> MATRLDRLVTILETGSTRLIRDTAVNQLADWQKQHPEELFNLLSRVVPYLRHKDWETRTTAAKAIGKIIENAPLYDPNAGQDEAAPEPTNGSFEVKKEEEKDVLEQDNFFRLESLDVATIVKYGRPLLRGGPVDYNLAALDPQKRLAHLKKTLNGRLGLLGRVFEDEEMPVEQIASPITPNDAAGANGVGRQDGASNDNQSQAIDESKMSARQLNVLKRKRKREAQKAAQGKSGFGDLSLRRSTTAGSDAFGEDTPMPDADSKKNKLAEYFSLDRPENTEEDTKIVSEFKGPVLPIKSEIEADDSLEGAEWPFERLCEFLKVDLFDPQWETRHGAAMGLREVIRVHGAGAGRRRGKTRKENNDLNRQWLDDLAYRLLCVLMLDKFTDYSSDTSVAPIRETVGQTLGAVLRHISVESVHAIYRLLYCMVTQEDLPSEQNMWAVCHGGMVGLRYVVAVRKDLLLQDGDMIDGVVRCVMQGLGDIDDDVRSVSAATLIPMAKEFVMMRRSALDSLINIVWESLSNLGDDLSASTGKIMDLLATLCSFPEVLEAMKVSASQDEERSFTLLVPRLYPFLRHTITSVRLAVLKALMTFANLGGETSQGWLNGRILRLIFQNIIVERDQDTLNMSLELWTTLVRRLAARDPAILADEFEAHAEPMMQLALHPIGVPRHPIPMNPALFQKPSGGTYSLPGASQTNSRRSSPPEGERATKRRRKSTKAEDVAPSTHTHDVDGHMIQGEVDLVGVDVLIRSRISAAKAMGLIMSFIPTPRLASYDTAVLQALSSPYASTQLAAAMVIDEYAKNCSTPEVASRFIEPLQKIIDLERPSHYRDLVTYVQRVRSASQQLINLFRDHGKVSQGKLPTLAVVVQGEPEAGPGAFSIANAEKVVNEDFERLKRLMAPGQRLIALPQLNEAREQTVEVIEEAKAAKEARDARIKAAAACALVAMKVLPKKPSPLIKAIMDSIKTEENQELQSRSAATIARLVQLFTESGRRGPAEKVVANLVKFSCVEVAETPEFPIHAHKTNVILSMQKEEDRVDHPDAVKYAREAKAARITRRGAKEALEILSKNFGAELLERVPTLRTFMEEPLVRAFSGDLPPEARDPENAFGQEIVDAMSVIRTMTPTLHPALHPFVMQQVPLVIKALRSDLSVFRYMAAKCMATICSVITVDGMTALVEKVLPSINNPLDLSFRQGAIEVIYHLIAVMGDAILPYVIFLIVPVLGRMSDSDNQIRLIATTSFATLVKLVPLEAGIPDPPGLSEELLKGRDRERTFIAQLLDPKKIEPFKIPVAIKAELRSYQQEGVNWLAFLNKYHLHGILCDDMGLGKTLQTICIVASDHHQRAEEFARTGAPEVRKLPSLIICPPTLSGHWQQEIKTYAPFLTVTAYVGSPAERRAMKDSLDKTDIVITSYDVCRNDIDVIEKYNWNYCVLDQGHLIKNPKAKITLAVKRLTSNHRLILTGTPIQNNVLELWSLFDFLMPGFLGAEKVFLDRFAKPIANSRYSKASSKEQEAGALAIEALHKQVLPFLLRRLKEEVLNDLPPKILQNYYCDLSDLQRKLFEDFTKREGKKITETAGRDDKEAKQHIFQALQYMRKLCNSPALVMKPGHKAYEDTQKYLAKHGTTLEDPIHAPKLGALRDLLVDCGIGVEGQESSDPLYTPIKPHRALIFCQMKEMLDMVQNTVLKQMLPSVSYLRLDGSVEANKRQDIVNKFNSDPSYDVLLLTTSVGGLGLNLTGADTVIFVEHDWNPQKDLQAMDRAHRIGQKKVVNVYRIITRGTLEEKILSLQRFKIDVASTVVNQQNAGLATMDTDQILDLFNLGESGPSLITDNKESIELEVLFQGPHHHHHHHH

The single subunit remodeler Mot1 (Modifier of transcription 1) is a Swi2/Snf2 enzyme that either activates or represses transcription in a context-dependent manner by dissociating TATA box-binding protein (TBP) and Negative Cofactor 2 (NC2) from promoter DNA. The N-terminal domain (Mot1NTD) recognizes TBP while the C-terminal domain (Mot1CTD) contains the catalytic Swi2/Snf2 ATPase that binds the DNA upstream from the TATA box. Swi2/Snf2 ATPases are members of the NTP-dependent helicase/translocase superfamily 2 (SF2) and are well known as the principal ATP hydrolyzing ‘engines’ of chromatin remodelers that govern processes such as transcription, replication, and DNA repair. Mot1 is an essential Swi2/Snf2 enzyme in yeast and the Mot1-TBP-NC2 regulatory axis is highly conserved in eukaryotes.

We determined the structure of this construct (residues 1–1836, Mot1∆C) harboring a point mutation in the Walker B motif (E1434Q) by Se-SAD to 3.2 Å. The construct covers the entire Mot1NTD and Mot1CTD domains but lacks 50 amino acids from the C-terminus. The CtMot1 enzyme is a ring-shaped protein. It forms a ring-like structure in which the substrate-interacting HEAT repeat ‘arch’ binds both lobes of the ATPase domain from opposing sites. Lobe 1 of the CtMot1CTD contacts the C-terminus of CtMot1NTD via HR16, a small insertion within HR12, and a ~ 45 amino acids linker. The tip of subdomain 1B interacts with HR1, thus lobe 1 effectively closes the ring structure of CtMot1. Lobe 2 binds the cleft between lobe 1 and HR1/2. Indeed, comparison of CtMot1CTD to other SF2 enzymes shows that lobe 2 is flipped ~180° from an ‘active’ conformation in which the ATPase and DNA-binding motifs would be properly aligned, that is lobe 1’s motifs I-III are properly situated in the ATP-binding cleft, while lobe 2’s motifs IV-VI are situated on the outside and are fully solvent-exposed. Although the precise orientation of lobe 2 might be additionally determined by the bridge element that is missing in the structure, our structural data suggest that the auto-inhibited resting state of CtMot1 is stabilized by the interactions between subdomain 2A and HR1/2. The bridge was almost entirely omitted from our crystallization construct and the only included residues (1822 –1836) together with the C-terminal expression tag are not visible in the electron density maps.>GSAHRFPALTQEQKKELSEIAQSIVANGKGILAADESVGTMGNRLQRIKVENTEENRRQFREILFSVDSSINQSIGGVILFHETLYQKDSQGKLFRNILKEKGIVVGIKLDQGGAPLAGTNKETTIQGLDGLSERCAQYKKDGVDFGKWRPVLRIADQCPSSLAIQENANALARYASICQQNGLVPIVEPEVIPDGDHDLEHCQYVTEKVLAAVYKALNDHHVYLEGTLLKPNMVTAGHACTKKYTPEQVAMATVTALHRTVPAAVPGICFLSGGMSEEDATLNLNAIN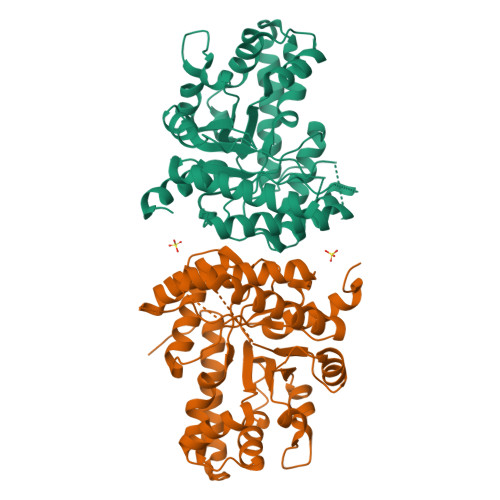LCPLPKPWKLSFSYGRALQASALAAWGGKAANKEATQEAFMKRAMANCQAAKGQYVHTGSSGAASTQSLFTACYTY[8x]> MPFVNKQFNYKDPVNGVDIAYIKIPNAGQMQPVKAFKIHNKIWVIPERDTFTNPEEGDLNPPPEAKQVPVSYYDSTYLSTDNEKDNYLKGVTKLFERIYSTDLGRMLLTSIVRGIPFWGGSTIDTELKVIDTNCINVIQPDGSYRSEELNLVIIGPSADIIQFECKSFGHEVLNLTRNGYGSTQYIRFSPDFTFGFEESLEVDTNPLLGAGKFATDPAVTLAHELIHAGHRLYGIAINPNRVFKVNTNAYYEMSGLEVSFEELRTFGGHDAKFIDSLQENEFRLYYYNKFKDIASTLNKAKSIVGT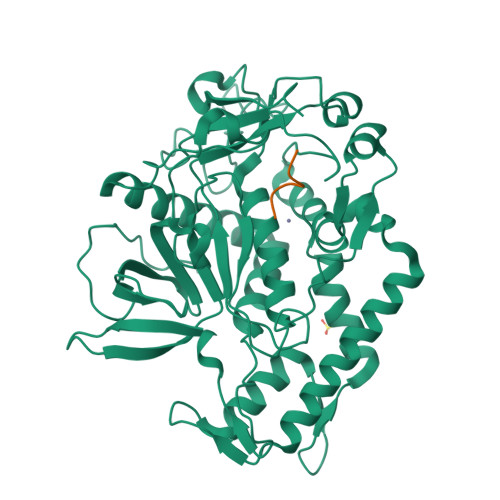TASLQYMKNVFKEKYLLSEDTSGKFSVDKLKFDKLYKMLTEIYTEDNFVKFFKVLNRKTYLNFDKAVFKINIVPKVNYTIYDGFNLRNTNLAANFNGQNTEINNMNFTKLKNFTGLFEHHHHHH;> QRATKMX>MSRLVLLVNPNKVHPPIAPYALDVLTTALEDEGFEVEVLDLTFRRDDWKTCLHEYFAERSPMLVGVTVRNTDTVYAFEQRPFVGEHREIITEIRRLTDAPVVGGGIGFSTMPFALVEYFGIEYGVKGPGEKILCELATAISEGRDTAGIPGLIRNTE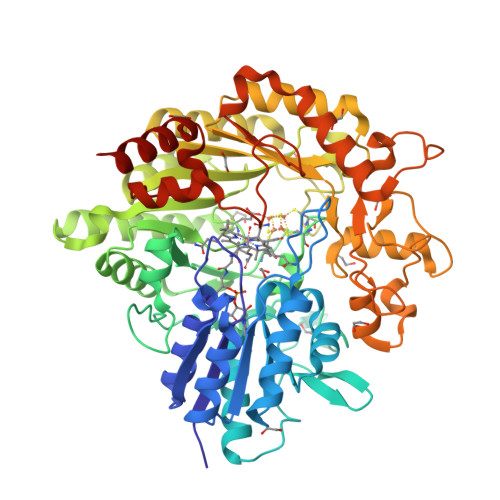RGAVRVPPAVLTVRHGKTQPAEPTGQFEPRVWQVDQLSVYRRRSGVPRKVDNLEYYRRGGLGSILTKNGCAYRCSHCVEPDAKGTRYGQRELASVVDEMESLAAQGILDQHTTDSEFNLSIAHAKNLLREIVRRRHADPDNPLNRLRLWVYCQPSPFDEEFADLLAAAGCRGVNVGSDHIRPELLSGWKVTEKGGTYYTFEDTERLVRLCRERGILTMVEALFGMPGETPETVRACVDAFMALDATVTGFSLGLRLFPYTPMGIEIAEQCAGVRTAPGLQSNTADGPIVLKPLRMCASPAEYERQFMFDEHGNFRLVCYFSPGLLPDPARAADPEERWHGAVADLWALIDPADHHRVMLPTVEGMSEHDNNYADNPFLTSLGGLGYTGAFWSHWRGREEIMRKAREAAAQSSHLPTPV[2x]> MSFLPS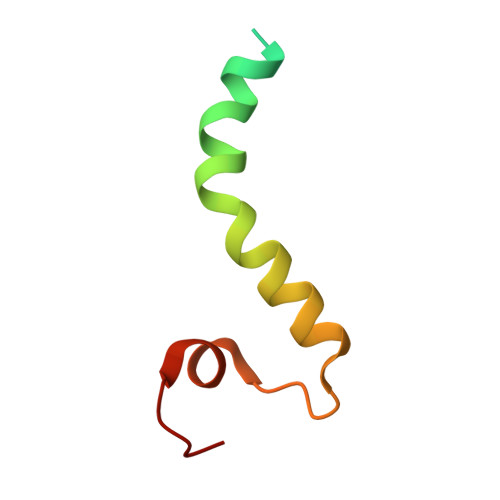FILSDESKERISKILTLTHNVAHYGWIPFVLYLGWAHTSNRPNFLNLLSPLPSV> GPLGSMSAAIAKPSAKPSAHVDPKSAPLKEIPDVLVDPRTMKRYMRGRFLGKGGFAKCYEITDMDTKEVFAGKVVPKSMLLKPHQKEKMSTEIAIHKSLDNPHVVGFHGFFEDDDFVYVVLEICRRRSLLELHKRRKAVTEPEARYFMRQTIQGVQYLHNNRVIHRDLKLGNLFLNDDMDVKIGDFGLATKIEFDG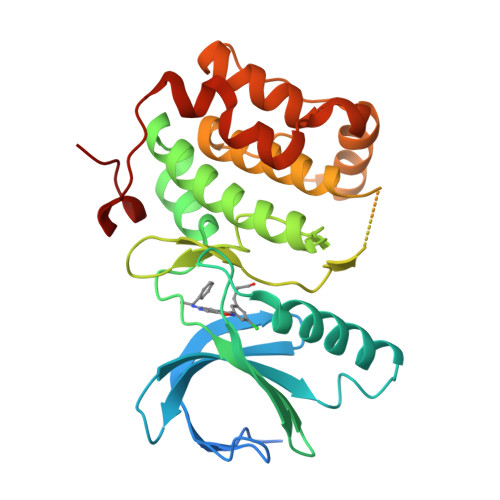ERKKDLCGTPNYIAPEVLCKKGHSFEVDIWSLGCILYTLLVGKPPFETSCLKETYIRIKKNEYSVPRHINPVASALIRRMLHADPTLRPSVAELLTDEFFTSGYAPMRLPTSCLTVPPRFS3-{[(Z)-1-carboxy-2-phenylethenyl]oxy}-2-hydroxybenzoic acid 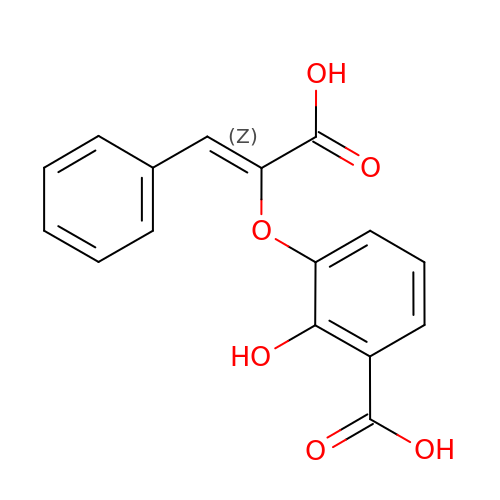| C16 H12 O6 | GJZVTQNBNWGGSJ-LCYFTJDESA-N3-[2-amino-6-(2-methylphenyl)quinolin-3-yl]-N-cyclohexylpropanamide | C25 H29 N3 O | 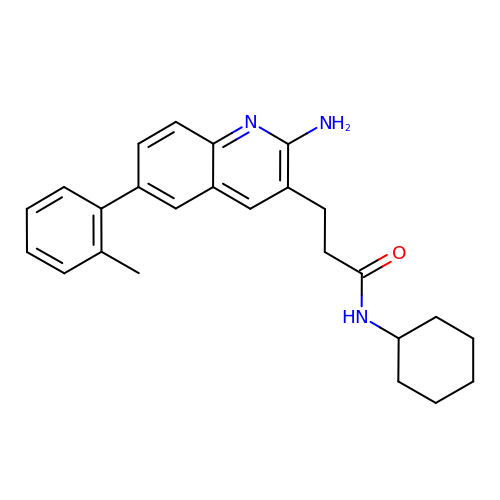JBOWUKRDBGMOJZ-UHFFFAOYSA-N> GSHMQKNPTVEYNQPAAPLQTKAPFSGAGPAASVPAGAPNEAQPGQSFEQWRDAFRQQALAGGIDAQTFDRAFAGVQPDPAVVEADRSQPEFTRPVWKYLEGALDPLRVRQGQARLAQHARILGEVDARYAVDADAVVAIWGMESNYGSHMGNKNVIRSLATLAYEGRRP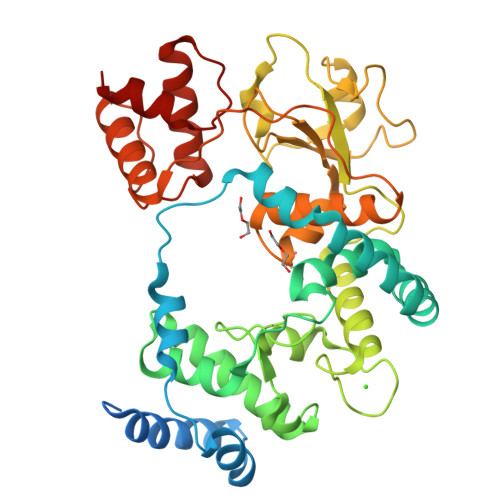EFAHAQLLAALKILQHGDVPASFMIGSWAGAMGQTQFIPTTHNQYAVDFDGDGKRDIWGSPGDALASTANYLKASGWIAGQPWGFEVRLPAGFDYSLAELTIRKPLGEWQGMGVQGVNGGPLPSGLSGEQASLLLPAGHRGPAFLVLHNFRAILKYNNSSAYALAVGLLADSFKGGGRIVGAWPLEDVPLSRSQRIELQRQLAARGHDPGAVDGIIGANTRKAIRACQQEFGWPADGYPTPALLDRLRTP>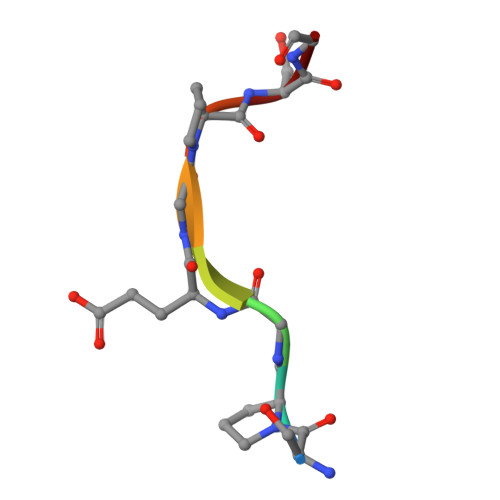 SPGEGPSG P-(2'-IODO-5'-THENOYL)HYDROTROPIC ACID | C14 H11 I O3 S | 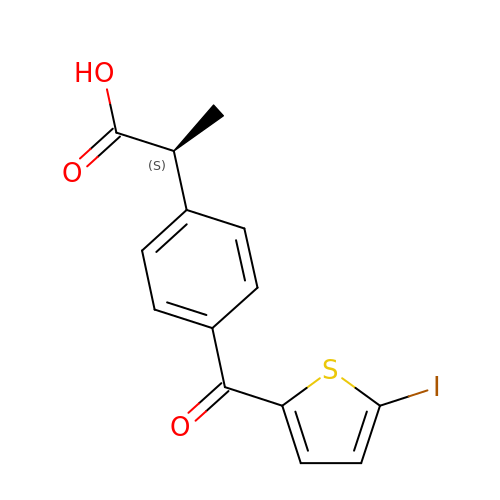UIZPHGUBGPJBAR-QMMMGPOBSA-N> MERNKLARQIIDTCLEMTRLGLNQGTAGNVSVRYQDGMLITPTGIPYEKLTESHIVFIDGNGKHEEGKLPSSEWRFHMAAYQSRPDANAVVHNHAVHCTAV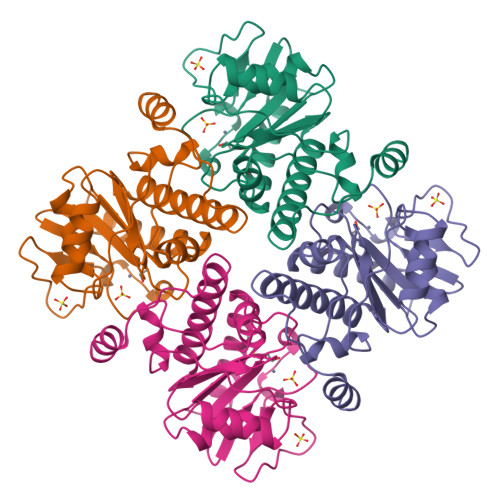SILNRSIPAIHYMIAAAGGNSIPCAPYATAGTRELSEHVALALKNRKATLLQHHGLIACEVNLEKALWLAHEVEVLAQLYLTTLAITDPVPVLSDEEIAVVLEKFKTYGLRIEE>GSSGMETTQTLRFKTKALAVLSKCYDHAQTHLKGGVLQVNLLSVNYGGPRLAAVANAGTAGLISFEVSPDAVAEWQNHQSPEEAPAAVSFRNLAYGRTCVLGKELFGSAVEQASLQFYKRPQGGSRPEFVKLTMEYDDKVSKSHHTCALMPYMPPASDRLRNEQMIGQVLLMPKTASSLQKWARQQGSGGVKVTLNPDLYVTTYTSGEACLTLDYKPLSVGPYEAFTGPVAKAQDVGAVEAHVVCSVAADSLAAALSLC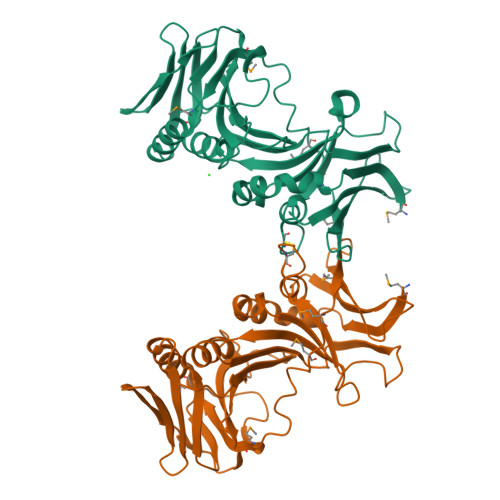RIPAVSVPILRFYRSGIIAVVAGLLTSAGDLPLDLSVILFNHASEEAAASTASEPEDKS[8x]> GSPQMSSLGTVDAPNFIVGNPWDDKLIFKLLSGLSKPVSSYPNTFEWQCKLPAIKPKTEFQLGSKLVYVHHLLGEGAFAQVYEATQGDLNDAKNK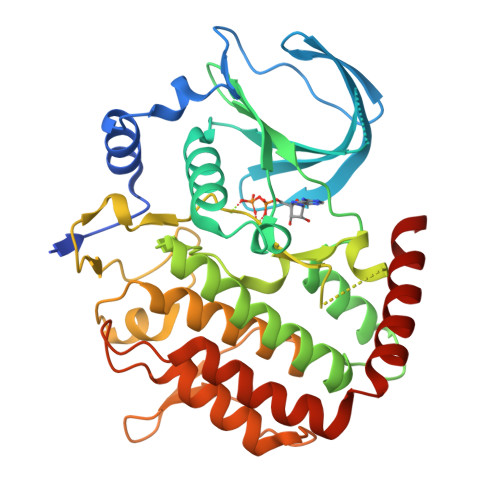QKFVLKVQKPANPWEFYIGTQLMERLKPSMQHMFMKFYSAHLFQNGSVLVGELYSYGTLLNAINLYKNTPEKVMPQGLVISFAMRMLYMIEQVHDCEIIHGDIKPDNFILGNGFLEQDDEDDLSAGLALIDLGQSIDMKLFPKGTIFTAKCETSGFQCVEMLSNKPWNYQIDYFGVAATVYCMLFGTYMKVKNEGGECKPEGLFRRLPHLDMWNEFFHVMLNIPDCHHLPSLDLLRQKLKKVFQQHYTNKIRALRNRLIVLLLECKRSRK> GPHMDLSELERDNTGRCRLSSPVPAVCRKEPCVLGVDEAGRGPVLGPMVYAICYCPLPRLADLEALKVADSKTLLESERERLFAKMEDTDFVGWALDVLSPNLISTSMLGRVKYNLNSLSHDTATGLIQYALDQGVNVTQVFVDTVGMPETYQARLQQSFPGIEVTVKAKADALYPVVSAASICAKVARDQAVKKWQFVEKLQDLDTDYGSGYPNDPKTKAWLKEHVEPVFGFPQFVRFSWRTAQTILEKEAEDVIWEDSASENQEGLRKITSYFL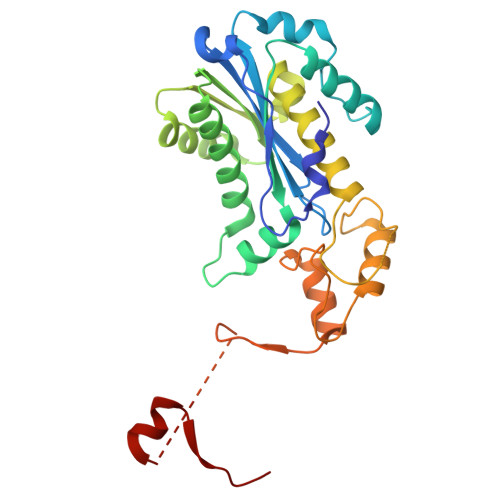NEGSQARPRSSHRYFLERGLESATSL1-chloronaphthalene 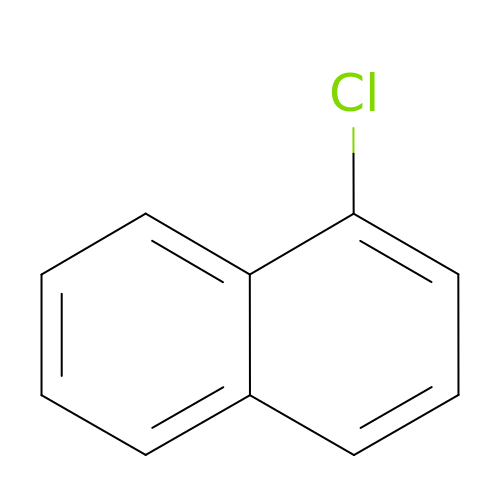| C10 H7 Cl | JTPNRXUCIXHOKM-UHFFFAOYSA-N> 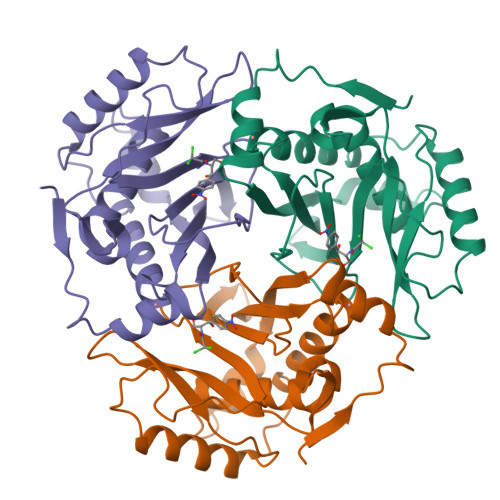MNYTKFDVKNWVRREHFEFYRHRLPCGFSLTSKIDITTLKKSLDDSAYKFYPVMIYLIAQAVNQFDELRMAIKDDELIVWDSVDPQFTVFHQETETFSALSCPYSSDIDQFMVNYLSVMERYKSDTKLFPQGVTPENHLNISALPWVNFDSFNLNVANFTDYFAPIITMAKYQQEGDRLLLPLSVQVHHAVCDGFHVARFINRLQELCNSKLK> STMEQLSQYLQEALHREQMLEQKLATLQRLLAITQEASDTSW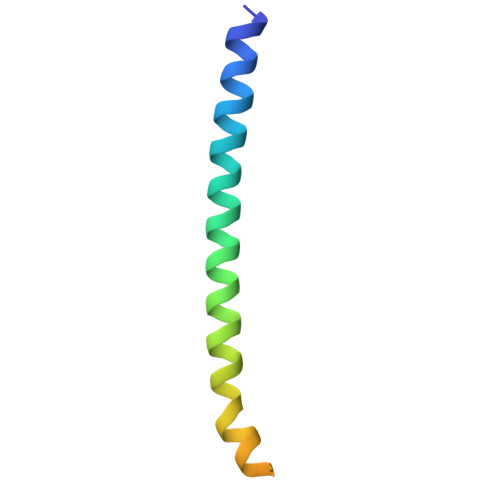QALIDEDRLLSRLEVMGNQLQA>MNLKDKILGVAKELFIKNGYNATTTGEIVKLSESSKGNLYYHFKTK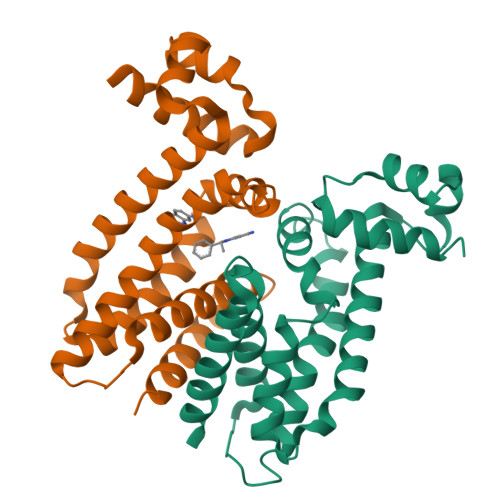ENLFLEILNIEESKWQEQWKKEQIKCKTNREKFYLYNELSLTTEYYYPLQNAIIEFYTEYYKTNSINEKMNKLENKYIDAYHVIFKEGNLNGEWSINDVNAVSKIAANAVNGIVTFTHEQNINERIKLMNKFSQIFLNGLSKHHHHHH[4x]> MSLRRGIYHIENAGVPSAIDLKDGSSSDGTPIVGWQFTPDTINWHQLWLAEPIPNVADTFTLCNLFSGTYMDLYNGSSEAGTAVNGWQGTAFTTNPHQLWTIKKSSDGTSYKIQNYGSKTFVDLVNGDSSDGAKIAGWTGTWDEGNPHQKWYFNRMSVSSAEAQAAIARNPHIHGTYRGYILDGEYLVLPNATFTQIWKDSGLPGSKQREQIYDCDDFAIAMKAAVGKWGADSWKANGFAIFCGVMLGVNKAGDAAHAYNFTLTKDHADIVFFEPWNGGYLNDIGYDSYMAFY

The Marasmius oreades agglutinin (MOA) is the holotype of an emerging family of fungal chimerolectins and an active Ca2+/Mn2+-dependent protease, which exhibits a unique papain-like fold with special active site features. While acting as a dimerization domain, the papain-like domain of MOA retains the characteristic L-/R-domain partition of PLCPs. As additional feature, the MOA dimer carries two binuclear metal-binding clusters, symmetrically placed at the dimerization interface (Grahn et al., 2009). MOA requires the presence of calcium or manganese (II) to switch from the inactive form to an active protease (Cordara et al., 2011, Wohlschlager et al., 2011).

Compared to papain, MOA exhibits a positional and functional swap of a glutamine and a tryptophan residue (Gln19/Trp177 in papain, and Trp208/Gln276 in MOA). To explore the significance of the structure-functional swap, we generated and tested the activity and thermal stability of both single- and double-site MOA variants targeting positions 208 and 276. The single-site substitution of Trp208 or Gln276 to either Ala (W208A, Q276A) or its papain counterpart (W208Q, Q276W) led to a partial loss of the enzymatic activity and decreased thermal stability. A MOA variant where Trp208 and Gln276 were both changed to their PLCP substitutes (W208Q/Q276W) completely lacked proteolytic activity and also had lower thermal stability than the wild-type enzyme. The side chains of both residues are relatively poorly defined by electron density and exhibit higher B-factors than in the MOA wild-type structure. The catalytic cysteine (Cys215) can be modeled in two different conformations, oriented approximately 90° apart. In the crystal structure of the double mutant, the Cys215 thiol group was found to be chemically modified to arsenocysteine. The formation of an arsenocysteine has previously been reported for other thiol-based enzymes (DeMel et al., 2004, Winger et al., 2008), and is a consequence of the reaction of cysteine with cacodylate, which was used as buffering agent in the crystallization conditions. However, simply substituting both Trp208 and Gln276 for their papain counterparts in variant W208Q/Q276W was insufficient to preserve enzyme activity.>[2x]MAAHQLSDFQRNKILRVFNTFYDCNHDGVIEWDDFELA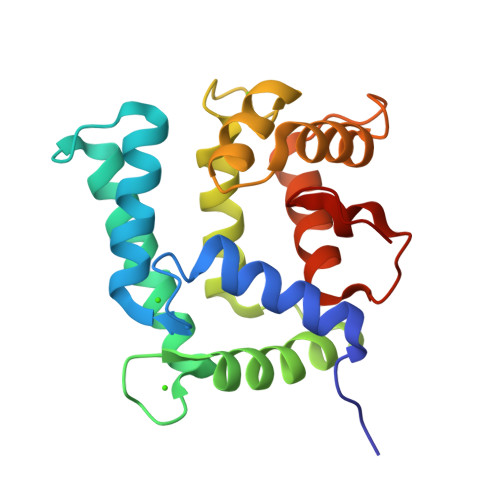IKKICNLHSWPTDGKKHNEARATLKLIWDGLRKYADENEDEQVTKEEWLKMWAECVKSVEKGESLPEWLTKYMNFMFDVNDTSGDNIIDKHEYSTVYMSYGIPKSDCDAAFDTLSDGGKTMVTREIFARLWTEYFVSNDRGAKGNHLFGTLKL Bacterial hybrid malic enzymes (MaeB grouping, multidomain) catalyse the transformation of malate to pyruvate, and are a major contributor to cellular reducing power and carbon flux. Distinct from other malic enzyme subtypes, the hybrid enzymes are regulated by acetyl-CoA, a molecular indicator of the metabolic state of the cell. The larger ME isoforms (hybrid enzymes) are predicted to be a fusion of two unrelated enzymes; a catalytic N-terminal ME subunit and a C-terminal phosphotransacetylase (PTA) domain. The PTA domain is homologous to PTA enzymes (that interconvert acetyl-CoA and phosphate to CoA and acetyl phosphate), yet they appear to lack critical catalytic residues and thus acts as a sensor instead.

We solved the crystal structure, to 1.67 Å, of the first 434 amino acids of MaeB, corresponding to the N-terminal catalytic domain (MaeBME). Structurally, MaeBME closely resembles the fold of small prokaryotic MEs, which form a tightly interacting dimer where the catalytic site is composed of residues from both protomers. Dimerisation in solution was confirmed by size-exclusion chromatography. MaeBME can be divided into three subdomains: region d1 which contains a Rossmann-like fold that forms the nucleotide binding site; region d2 which is mixed α/β and contains an N-terminal extension that sits over the dimer interface and extends into the opposing monomer; and a small “hook-like” subdomain (residues 369–386) that has no structural equivalent in other characterised ME folds and is best-described as a projecting loop with central alpha helix. Comparatively, the hook region is easily discerned as an insert in the primary sequence of hybrid MEs, and packs against d1 via several conserved hydrophobic residues. Each of these catalytic residues is in an equivalent pose to those from the eukaryotic enzymes, with the difference that Y52 is contributed from the other monomer rather than on the same chain. Our truncated ME construct (MaeBME) retained activity, but was insensitive to inhibition by acetyl-CoA, CoA and acetyl phosphate, confirming that these allosteric inhibitors act at the appended PTA domain.

>[2x]MGSSHHHHHHSMDNKTETKIEPKTGTTNFDQEALLYHQQGKPGKIEVISSKPCATEKDLSLAYSPGVAAPCKAIAKDPAKVYDYTAKGNLVAVISNGTAVLGLGNIGPAAGKPVMEGKGILFKQFAGIDVFDIEVAATDVDVFCNAVRVLEPTFGGINLEDIKAPECFEIEERLKKEMNIPVFHDDQHGTAIVSGAALLNACSITNRKMETVRIVVNGAGASANSCAKIFIALGARRENIIMCDSQGVIYKGRTAGMNKYKEYFASETEARTLTEALRGADVFVGLSVAGALTPEMLKDMAKDPIIFAMANPEPEITPDKARAARPDAIIATGRSDYPNQVNNVLGFPSIFRGALDTRSTQINEEMKLAAVHALAKLAREDVPDKVSATYGGKSFKFGRDYLIPKPFDTRVLLWVAPEVAKAAMKSGVATRAIEDWDQYRESLEA>MIPDVSQALAWLEKHPQALKGIQRGLERETLRVNADGTLATTGHPEALGSALTHKWITTDFAEALLEFITPVDGDIEHMLTFMRDLHRYTARNMGDERMWPLSMPSYIAEGQDIELAQYGTSNTGRFKTLYREGLKNRYGALMQTISGVHYNFSLPMAFWQAKSGDISGADAKEKISAGYFRVIRNYYRFG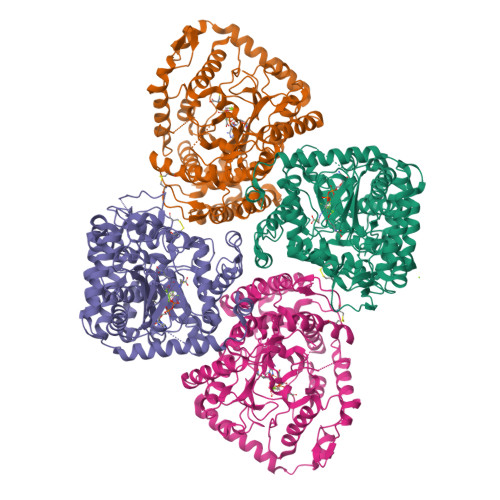WVIPYLFGASPAISSSFLQGKPTSLPFEKTESGMYYLPYATSLRLSDLGYTNKSQSNLGITFNDLYEYVAGLKQAIKTPSEEYAKIGIEKDGKRLQINSNVLQIENELYAPIRPKRVTRSGESPSDALLRGGIEYIEVRSLDINPFSPIGVDEQQVRFLDLFMVWCALADAPEMSSSELACTRVNWNRVILEGRKPGLTLGIGCETAQFPLPQVGKDLFRDLKRVAQTLDSINGGEAYQKVCDELVACFDNPDLTFSARILRSMIDTGIGGTGKAFAEAYRNLLREEPLEILREEDFVAEREASERRQQEMEAADTEPFAVWLEKHA[4x]>MNGPKADIAWAASAEVANKPRLVFVGDELRYAQGANQRDVELDGFVNYHWLTSPGGLGLPKVMLEAGINAPAEVVGPDRSRRALIAIRSSPWKAGHETNPWHDEFDLDHGHVRYFGDHKPSTVGLPGETKGNRLLLEAARLHAGTTREERLLAPPLFLFRAVTVHRAGRAVVKGHVEFCGAAIIERLEHVVQRDPETGRSFPNLSLDLAVVSGGEIDGVDFRWIDDRRNAALAAGETLRHAPESWIRWVRQGRLAIPGIRRRVLASAVQSSKEQQPASGSAEAATLQTLYKFYDGRKHAFELLASRVAAEVFRESGARYKEGWLSRSSGDGGVDFIGRIDMGSLKASTP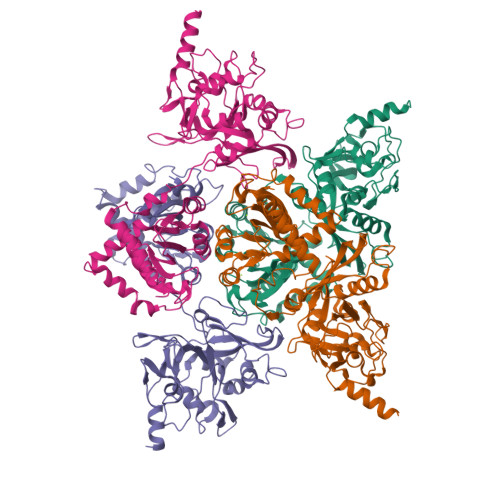VVVLGQAKCIQPTSSVSPEQVARVVARLRRGWIGVYVTTGSFSRQAQVEIIDDQYPVVLIAGGTLAATVRRMVQANYGGDLDALLASTVDEYGAAVTHRRPEEVISL[4x]> ETGQCRIQKCTTDFVSLTSHLNSAVDGFDSEFCKALRAYAGCTQRTSKACRGNLVYHSAVLGISDLMSQRNCSKDGPTSSTNP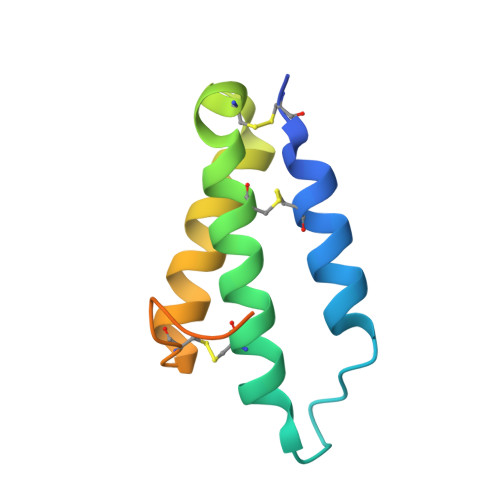EVTHGTKHHHHHH> CQPIFLNVLEAIEPGVVCAGHDNNQPDSFAALLSSLNELGERQLVHVVKWAKALPGFRNLHVDDQMAVIQYSWMGLMVFAMG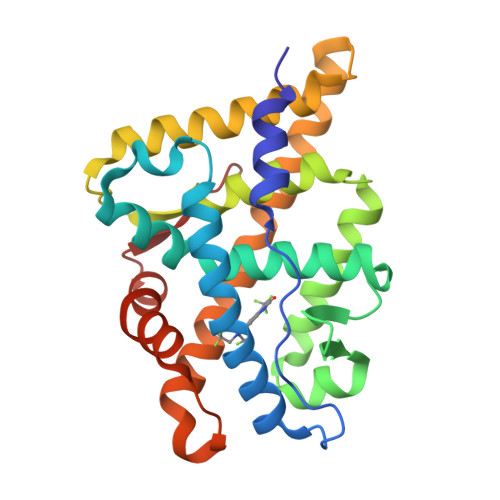WRSFTNVNSRMLYFAPDLVFNEYRMHKSRMYSQCVRMRHLSQEFGWLQITPQEFLCMKALLLFSIIPVDGLKNQKFFDELRMNYIKELDRIIACKRKNPTSCSRRFYQLTKLLDSVQPIARELHQFTFDLLIKSHMVSVDFPEMMAEIISVQVPKILSGKVKPIYFHT> GLGQMLESMIDNTVRETVGAATSRDALPNTEASGPTHSKEIPALTAVETGATNPLVPSDTVQTRHVVQHRSRSESSIESFFARGACVTIMTVDNSASTTNKDKLFAVWKITYKDTVQLRRKLEFFTYSRFDMELTFVVTANFTETNNGHALNQVYQIMYIPPGAPVPEKWDDYTWQTSSNPSIFYTYGTAPARISVPY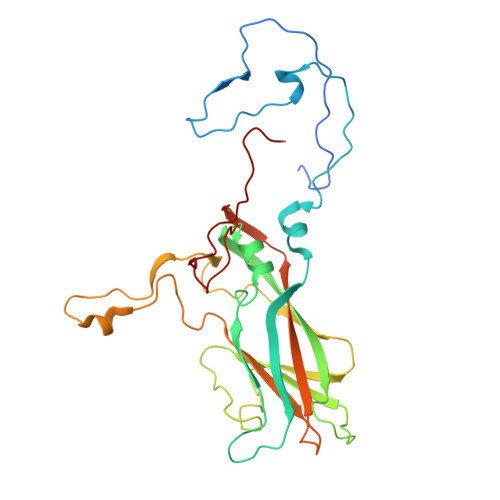VGISNAYSHFYDGFSKVPLKDQSAALGDSLYGAASLNDFGILAVRVVNDHNPTKVTSKIRVYLKPKHIRVWCPRPPRAVAYYGPGVDYKDGTLTPLSTKDLTTY>[2x]MDYKDDDDKENLYFQGMNGEAICSALPTIPYHKLADLRYLSRGASGTVSSARHADWRVQVAVKHLHIHTPLLDSERKDVLREAEILHKARFSYILPILGICNEPEFLGIVTEYMPNGSLNELLHRKTEYPDVAWPLRFRILHEIA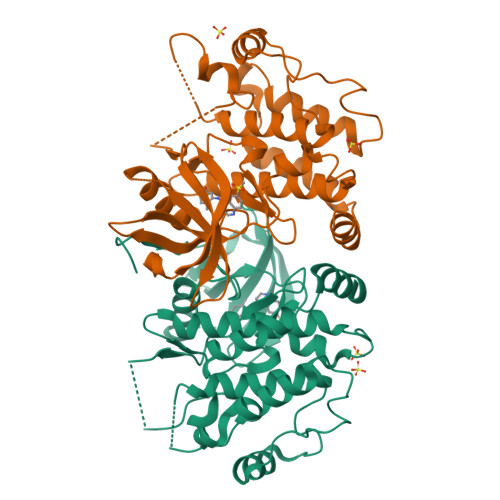LGVNYLHNMTPPLLHHDLKTQNILLDNEFHVKIADFGLSKWRMMSLSQSRSSKSAPEGGTIIYMPPENYEPGQKSRASIKHDIYSYAVITWEVLSRKQPFEDVTNPLQIMYSVSQGHRPVINEESLPYDIPHRARMISLIESGWAQNPDERPSFLKCLIELEPVLRTFEEITFLEAVIQLK>MGLENNQNCLQHRMGTTTIKLVAADGSPLANKEVTVKQTKHKFLFGCAEFTSVPYANNKFEGKQKEKIEERYEKFFDLFNFVTLPFYWGKFEPVKGKPDTESLKNAAKWLQTKGVELKGHPLCWHTETAPWLLDMSNSEIFSTQIKRIHRDVTDFKGLIDMWDVINEVVIMPIFDKYDNGITRICKDMGRIKLVREVFKAARESNPNATLLINDFETSESYDILIEGLLESGVHIDAIGIQSHMHQGYWGVEKTQEILERFSRFKLPIHFTENTLVSGHLMPPEIVDLNDYQIPEWPSTPEGEERQAQEAVTHYKTLFSHPLVEAITWWDFVDGGWLKAPSGFITQDNRVKPIYHALHDLIKNQWWTKPMDLI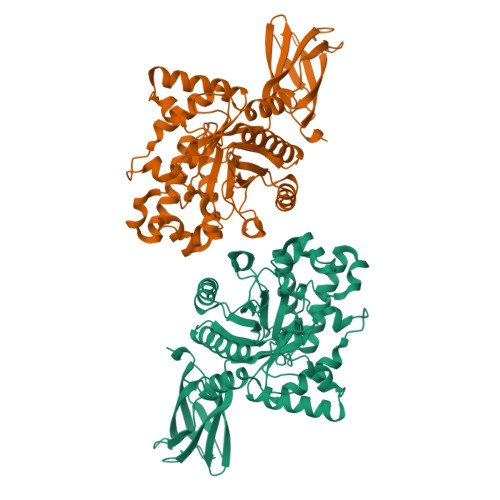SDENGLVNVSGFLGEYEVTFDGKSKSFCLDNNNETVTISA[2x]> GASKSHKCDFTKEKYLLSGEKEVSCEIDANPSDDITFICPNKIDSLCFHTVNISKNINQNKSTMSIQDLLYGSVVYGNTLFISPYVRTNTPFYCFCNLDTVTIQKFLKINRFLKDDDELSEADVMKHLKGGNVSEAQADEYLNKALNRFKKMKDLSKFFNDQADNTTKLNLPKSLNIPNDILNYDVYNSSNNRNDIVVKDEVTNKQIISKRGIMSVFVRSNNNVIKGCDFGNNNKNYFSHPISVAGKVNNKVCKIQGKPGELVGFKCAFEENGKVEPPNCFDQVLHKNKVTDLKTLIPGYASYTNKHSSKYPYYLKIPHFVNEQYTIQCKCKSNNSQNEYTFELDIQPGES;> GASNLTCDFNDVYKLEFHPNQQTSVTKLCNLTPNVLEKVTIKCGSDKLNYNLYPPTCFEEVYASRNMMHLKKIKEFVIGSSMFMRRSLTPNKINEVSFRIPPNMMPEKPIYCFCENKKTITINGSNGNPSSKKDIINRGIVEIIIPSLNEKVKGCDFTTSESTIFSKGYSINEISNKSSNNQQDIVCTVKAHANDLIGFKCPSNYSVEPHDCFVSAFNLSGKNENLENKLKLTNIIMDHYNNTFYSRLPSLISDNWKFFCVCSKDNEKKLVFTVEASISS

The 6-cysteine (6-cys) protein family is one of the most abundant surface antigens and expressed throughout the Plasmodium falciparum life cycle. This protein family is conserved across Plasmodium species and plays critical roles in parasite transmission, evasion of the host immune response and host cell invasion. On the merozoite surface, Pf12 is one of the most abundant GPI-anchored proteins and forms a heterodimeric complex with the secreted 6-cys protein Pf41 (Gilson et al. 2006, Taechalertpaisarn et al. 2012, Tonkin et al. 2013). However, Pf12 and Pf41 knockout parasites have no growth defects during the blood stages and polyclonal antibodies against either Pf12 or Pf41 showed no growth inhibition. Both Pf12 and Pf41 contain two 6-cys domains and the crystal structures of the individual proteins have been determined (Arredondo et al. 2012, Tonkin et al. 2013, Parker et al. 2015).

The Pf12-Pf41 crystal structure was determined at a resolution of 2.85 Å by molecular replacement and reveals a heterodimeric complex of approximately 80 × 65 × 35 Å in size. The asymmetric unit contained one Pf12 D1D2 and one Pf41 D1D2 molecule. Both proteins fold into two 6-cys domains (D1 and D2) adopting a β-sandwich fold with three disulfide bonds per domain. The last two β-strands of the Pf41 D1 domain are connected via a 110 amino acid long insertion, termed inserted-domain-like region (ID), which spans amino acids 115 to 225. The crystal structure of Pf12-Pf41 shows that both proteins interact through two distinct binding sites (Site 1 and Site 2) with a total surface area of 1051 Å2, with Site 1 and Site 2 contributing to the interaction surface with 578 Å2 and 473 Å2 respectively. Site 1 shows that the interdomain region of Pf12 forms contacts with the Pf41 D2 domain, with residues on both Pf12 domains interacting with extended loops on one side of the Pf41 D2 domain. Site 2 comprises of the Pf12 D2 domain in which its bottom β-sheet and surrounding loops form a concave protein surface that engages with the long α-helix of the Pf41 ID (and D bottom). H234 and H336 were mutated as they coordinate a cadmium ion at the Pf12-Pf41 interface, which we propose may feature a crystallization artefact rather than required for Pf12-Pf41 binding (Fig. 1Dtop). Important for the assembly of Pf12 and Pf41 is a π-π interaction involving Pf12 residue Y264 and Pf41 residue F337, and hydrophobic contacts between Pf12 F283 and Pf41 residues L159 and L163. Furthermore, a region of 33 residues spanning 84–116, which includes the β-sheets β5 to β7 of the Pf12 D1 domain, which was unstructured in the unbound Pf12 molecule, was well resolved in the presence of Pf41, suggesting that binding of Pf41 possibly reduces the flexibility within Pf12 and stabilises the junction of the Pf12 D1-D2 domains. Previous studies which used cross-linking approaches to develop a model of this heterodimeric complex showed a few differences from our Pf12-Pf41 crystal structure.> PNFSGNWKIIRSENFEELLKVLGVNVMLRKIYVAAASKYAVEIKQEGDTFYIKVSTTVYTTEINFKVGEEFEEQTVDGRPCKSLVKWESENKMVCEQKLLKGEGPKTSWTKELTNDGELIETMTADDVVC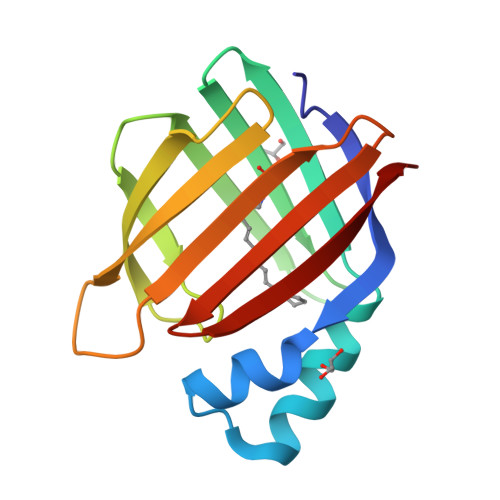TQVFVRE>MGSSHHHHHHSSGRENLYFQGHMAQNPERRAALVNAAIEVLAREGARGLTFRAVDVEANVPKGTASNYFPSRDDLFDQVGKRIHERLGPDPSVVEESGRKPQNLELAIEYMQGLFGRITRDRTGYLALQELRLEAVRRPELRTTLTRTISENLKRDIGFHLDSGLPGDRS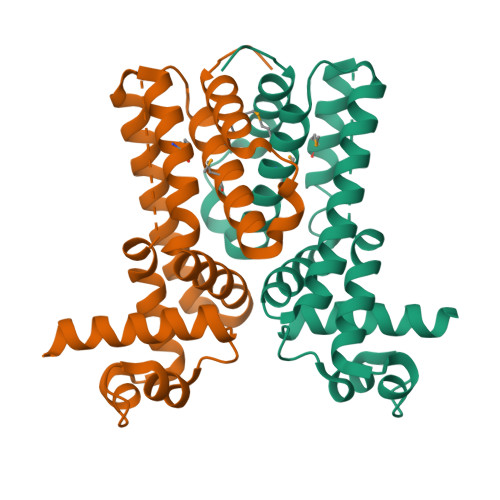TVLMLYLAMNALIVEHLTLPGVLEGVDTERLVADLVTRAVATPDA[4x]> MIDLAIGQVPIANWVSSATDWITSTFSSGFDVIQKSGTVLMNGITGALTAVPFWLMIAVVTILAILVSGKKIAFPLFTFIGLSLIANQGLWSDLMSTITLVLLSSLLSIIIGVPLGIWM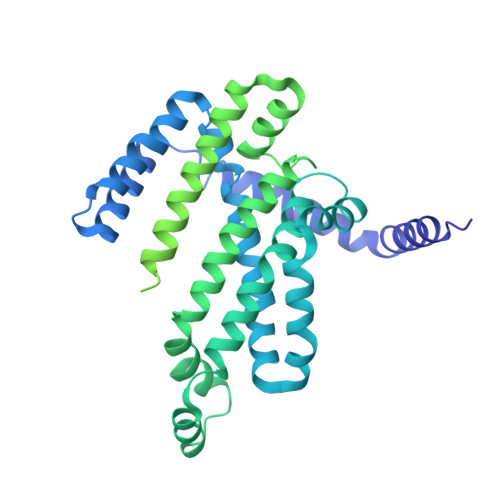AKSDLVAKIVQPILDFMQTMPGFVYLIPAVAFFGIGVVPGVFASVIFALPPTVRMTNLGIRQVSTELVEAADSFGSTARQKLFKLEFPLAKGTIMAGVNQTIMLALSMVVIASMIGAPGLGRGVLAAVQSADIGKGFVSGISLVILAIIIDRFTQKLNVSPLEKQGNPTVKKWKRGIALVSLLALIIGAFSGMSFGKTASDKKVDLVYMNWDSEVASINVLTQAMKEHGFDVKTTALDNAVAWQTVANGQADGMVSAWLPNTHKTQWQKYGKSVDLLGPNLKGAKVGFVVPSYMNVNSIEDLTNQANKTITGIEPGAGVMAASEKTLNSYDNLKDWKLVPSSSGAMTVALGEAIKQHKDIVITGWSPHWMFNKYDLKYLADPKGTMGTSENINTIVRKGLKKENPEAYKVLDKFNWTTKDMEAVMLDIQNGKTPEEAAKNWIKDHQKEVDKWFKGSIEGRHHHHHH> MHNHNHNHNHNHNGGENLYFQGASLTEIEHLVQSVCKSYRETCQLRLEDLLRQRSNIFSREEVTGYQRKSMWEMWERCAHHLTEAIQYVVEFAKRLSGFMELCQNDQ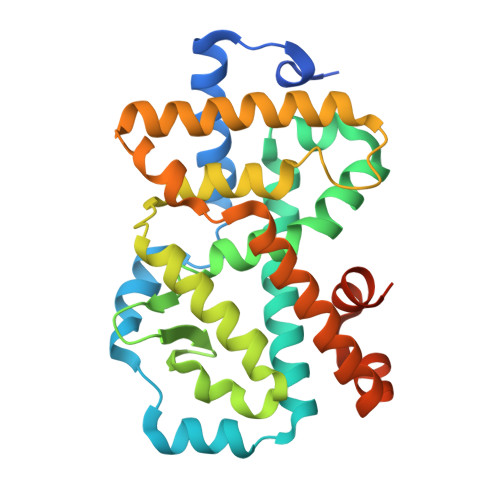IVLLKAGAMEVVLVRMCRAYNADNRTVFFEGKYGGMELFRALGCSELISSIFDFSHSLSALHFSEDEIALYTALVLINAHRPGLQEKRKVEQLQYNLELAFHHHLCKTHRQSILAKLPPKGKLRSLCSQHVERLQIFQHLHPIVVQAAFPPLYKELFSGGGKEKHKILHRLLQDSS>[4x]MRVLALSAVFLVASIIGMPAVAKEWQENKSWNAHFTEHKSQGVVVLWNENKQQGFTNNLKRANQAFLAASTFKIPNSLIALDLGVVKDEHQVFKWDGQTRDIATWNRDHNLITAMKYSVVPVYQEFARQIGEARMSKMLHAFDYGNEDISGNVDSFWLDGGIRISATEQISFLRKLYHN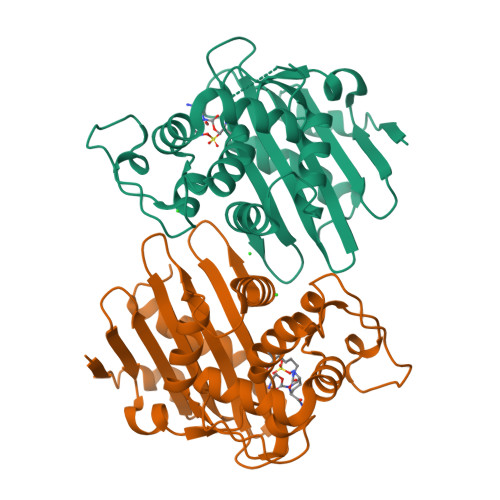KLHVSERSQRIVKQAMLTEANGDYIIRAKTGYSTRIEPKIGWWVGWVELDDNVWFFAMNMDMPTSDGLGLRQAITKEVLKQEKIIP> MRGSHHHHHHGSLSSSPSEILQELGKGSTHPQPGVSPPAAPAAPGPKDGPGETDAFGNSEGKELVASGENKIKQGLLPSLEDLLFYTIAEGQEKIPVHKFITALKSTGLRTSDPRLKECMDMLRLTLQTTSDGVMLDKDLFKKCVNSNIVLLTQAFRRKFVIPDFMSFTSHIDELYESAKKQSGGKVADYIPQLAKFSPDLWGVSVCTADGQRHSTGDTKVPFCLQSCVKPLKYAIAVNDLGTEYVHRYVGKEPSGLRFNKLFLNEDDKPHNPMVNAGAIVVTSLIKQGVNNAEKFDYVMQFLNKMAGNEYVGFSNATFQSERESGDRNFAIGYYLKEKKCFPEGTDMVGILDFYFQLCSIEVTCESASVMAATLANGGFCPITGERVLSPEAVRNTLSLMHSCGMYDFSGQFAFHVGLPAKSGVAGGILLVVPNVMGMMCWSPPLDKMGNSVKGIHFCHD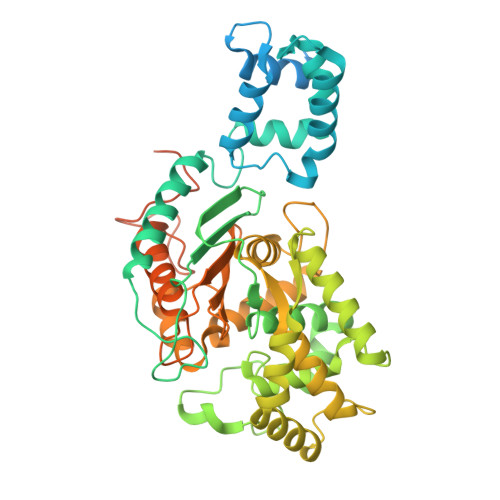LVSLCNFHNYDNLRHFAKKLDPRREGGDQRHSFGPLDYESLQQELALKETVWKKVSPESNEDISTTVVYRMESLGEKS> SILVRRDAAPGASKLRAVLEKLKLSRDDISTAAGMVKGVVDHLLLRLKCDSAFRGVGLLNTGSYYEHVKISAPNEFDVMFKLEVPRIQLEEYSNTRAYYFVKFKRNPKENPLSQFLEGEILSASKMLSKFRKIIKEEINDIKDTDVIMKRKRGGSPAVTLLISEKISVDITLALESKSSWPASTQEGLRIQNWLSAKVRKQLRLKPFYLVPKHAKEGNGFQEETWRLSFSHIEKEILNNHGKSKTCCENKEEKCCRKDCLKLMKYLLEQLKERFKDEEHLDKFSSYHVKTAFFHVCTQNPQDSQWDRKDLGLCFDNCVTYFLQCLRTEKLENYFIPEFNLFSSNLIDKRSKEFLTKQIEYERNNEFPVFDEF

Binding of dsDNA to cGAS activates the synthesis of c[G(2′,5′)pA(3′,5′)p], a diffusible cyclic dinucleotide referred to as cGAMP, which travels to and activates the endoplasmic reticulum membrane-anchored adaptor protein, stimulator of interferon genes (gene symbol STING/TMEM173). Activated STING recruits and activates TANK-binding kinase 1 (gene symbol TBK1), which in turn phosphorylates the transcription factor family of interferon regulatory factors (IRFs)10 inducing cytokine and type I interferon mRNA expression. Likewise, embryonic lethality caused by deficiency of Dnase2, an endonuclease responsible for degradation of excessive DNA in lysosomes during endocytosis, was completely rescued by additional knockout of Cgas24 or Sting25. These observations support cGAS as a drug target and inhibition of cGAS may provide a therapeutic strategy for preventing autoinflammation and treating diseases such as systemic lupus erythematosus (SLE) with involvement of anti-dsDNA antibodies. In summary, we developed a class of h-cGAS specific and potent small-molecule inhibitors active in primary human macrophages.

The placement of a methoxy group (G098) resulted in a 2-fold improvement for inhibition of h-cGAS but not m-cGAS, while the placement of a pyrazole group (G108) yielded a 4-fold improved IC50 value for h-cGAS to 27.5 nM but a 300-fold reduction to 5.15 µM for m-cGAS. To explore the structural basis for h-cGAS inhibition, we obtained crystals of G108 bound to h-cGASCD. During optimization of crystallization conditions, we realized that double substitution of amino acids K427E/K428E facilitated crystal packing and improved crystal quality and inhibitor occupancy substantially compared to wild-type apo h-cGASCD. The electron density in the 2Fo–Fc map (contoured at 1.2 σ) for bound G108 can be traced for the chlorine-substituted pyridoindole core and the pyrazole ring of the bound G108, but not for the hydroxyl-ethanone side chain attached to the non-planar six-membered ring, due to its apparent flexibility. The tricyclic pyridoindole core of bound G108 was sandwiched between the guanidinium group of Arg376 and the aromatic ring of Tyr436, while the pyrazole ring of bound G108 was anchored in a hydrophobic pocket lined by the side chains of His437, Phe488, and Leu490 of h-cGAS. The pyrazole ring of bound G108 formed a hydrogen bond with one water molecule in the binding pocket. However, we also observed a similar reduction for G108, which although it has the ability of hydrogen-bond by its pyrazole substituent was not as deeply inserted into the binding pockets of h-cGASCD to reach the Tyr248. At inhibitor concentrations of 10 µM, representing cellular IC90 or more for the inhibitors against cGAS pathway, only G108 showed weak off-target inhibition of the directly cGAMP-stimulated STING pathway and the hairpin-RNA (hpRNA) stimulated RIG-I pathway.2-[(1R,3S,5R,7S)-2-[4-(4-FLUOROPHENYL)PHENYL]-6-HYDROXYADAMANTAN-2-YL]-1-(3-HYDROXYAZETIDIN-1-YL)ETHAN-1-ONE | C27 H30 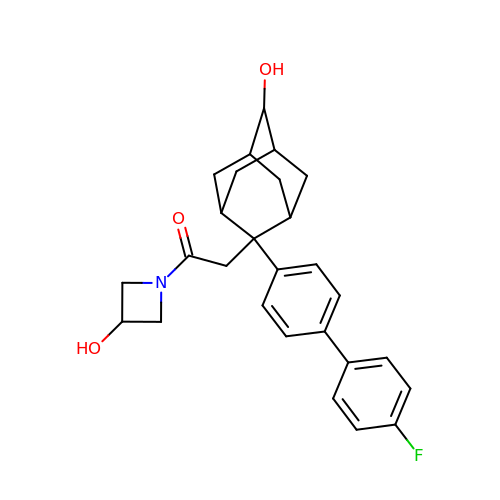F N O3 | FBTIGDUFOZJGFY-YRDUTZFVSA-N>[4x]MRKELVFVLLALFLCAGCNGNKKKMNGEHDLDAANITLDDHTISFYYNWYGNPSVDGEMKHWMHPIALAPGHSGDVGAISGLNDDIACNFYPELGTYSSNDPEIIRKHIRMHIKANVGVLSVTWWGESDYGNQSVSLLLDEAAKVGAKVCFHIEPFNGRSPQTVRENIQYIVDTYGDHPAFYRTHGKPLFFIYDSYLIKPAEWAKLFAAGGEISVRNTKYD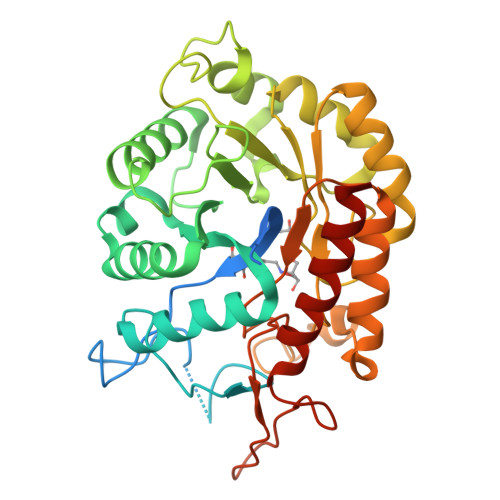GLFIGLTLKESELPDIETACMDGFYTYFAATGFTNASTPANWKSMQQWAKAHNKLFIPSVGPGYIDTRIRPWNGSTTRDRENGKYYDDMYKAAIESGASYISITSFNEWHEGTQIEPAVSKKCDAFEYLDYKPLADDYYLIRTAYWVDEFRKARSASEDVQ> GSMGKLSEQLKHCNGILKELLSKKHAAYAWPFYKPVDASALGLHDYHDIIKHPMDLSTV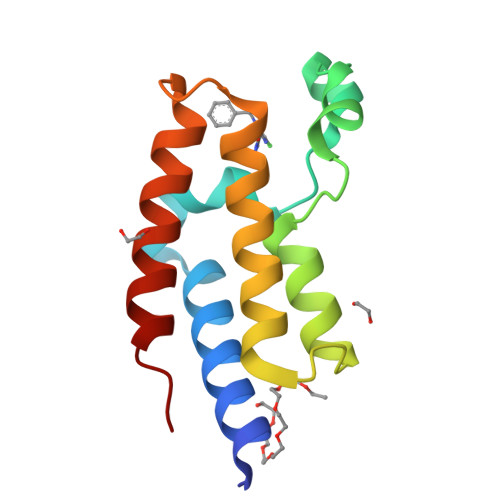KRKMENRDYRDAQEFAADVRLMFSNCYKYNPPDHDVVAMARKLQDVFEFRYAKMPD>MSK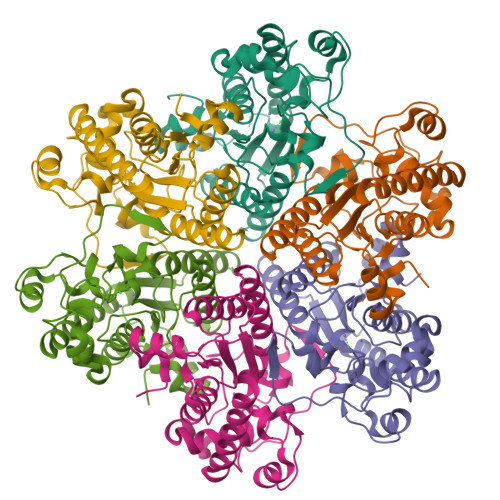SVFVGELTWKEYEARVAAGDCVLMLPVGALEQHGHHMCMNVDVLLPTAVCKRVAERIGALVMPGLQYGYKSQQKSGGGNHFPGTTSLDGATLTGTVQDIIRELARHGARRLVLMNGHYQNSMFIVEGIDLALRELRYAGIQDFKVVVLSYWDFVKDPAVIQQLYPEGFLGWDIEHGGVFETSLMLALYPDLVDLDRVVDHPPATFPPYDVFPVDPARTPAPGTLSSAKTASREKGELILEVCVQGIADAIREEFPPT[6x]>[3x]PVMHPHGAPPNHRPWQMKDLQAIKQEVSQAAPGSPQFMQTIRLAVQQFD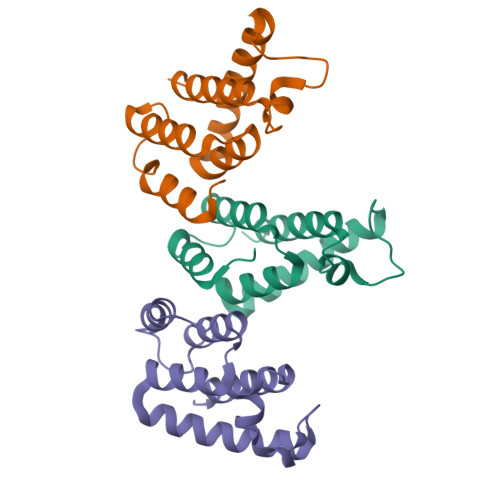PTAKDLQDLLQYLCSSLVASLHHQQLDSLISEAETRGITGYNPLAGPLRVQANNPQQQGLRREYQQLWLAAFAALP> EDGSDPPSGDFLTEGGGVRGPRLVERQQSACKETGWPFCSDEDWNTKCPSGCRMKGLIDEVDQDFTSRINKLRDSLFNYQKNSKDSNTLTKNIVELMRGDFAKANNNDNTFKQINEDLRSRIEILRRKVIEQVQRINLLQKNVRDQLVDMKRLEVDIDIKIRSCKGSCSRALEHKVDLEDYKNQQKQLEQVIAINLLPSRDIQYLPILKMSTITGPVPREFKSQLQEAPLEWKA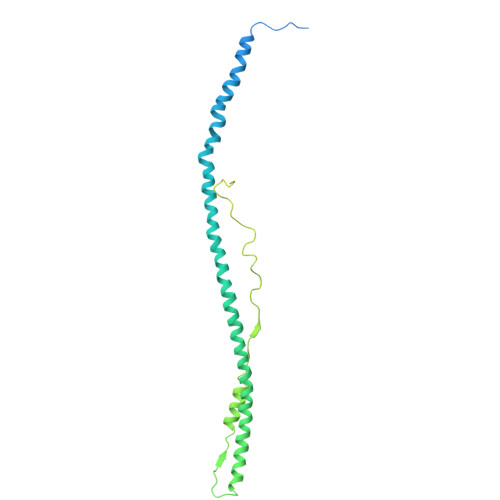LLEMQQTKMVLETFGGDGHARGDSVSQGTGLAPGSPRKPGTSSIGNVNPGSYGPGSSGTWNPGRPEPGSAGTWNPGRPEPGSAGTWNPGRPEPGSAGTWNPGRPEPGSAGTWNPGRPEPGSAGTWNTGSSGSSSFRPDSSGHGNIRPSSPDWGTFR9-AMINO-N-[3-(DIMETHYLAMINO)PROPYL]ACRIDINE-4-CARBOXAMIDE | C19 H22 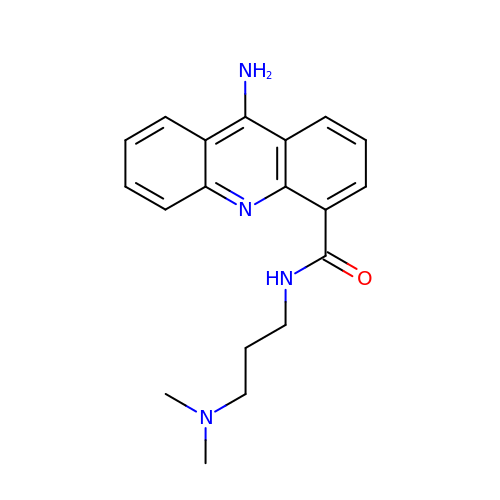N4 O | VNWAULKXOPRJEL-UHFFFAOYSA-N> MKLLTHNLLSSHVRGVGSRGFPLRLQATEVRICPVEFNPNFVARMIPKVEWSAFL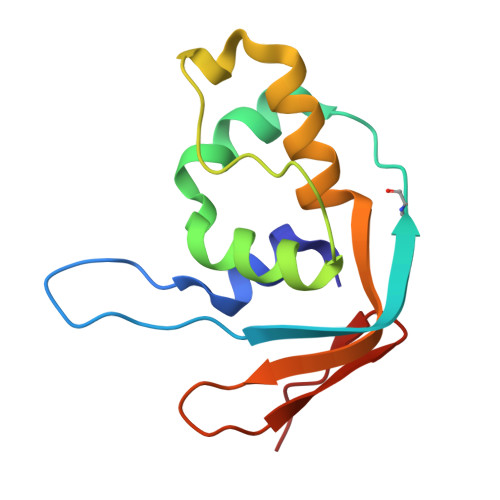EAADNLRLIQVPKGPVEGYEENEEFLRTMHHLLLEVEVIEGTLQCPESGRMFPISRGIPNMLL>MLRFVTKNSQDKSSDLFSICSDRGTFVAHNRVRTDFKFDNLVFNRVYGVSQKFTLVGNPTVCFNEGSSYLEGIAKKYLTLDGGLAIDNVLNELRSTCGIPGNAVASHAYNITSWRWYDNHVALLMNMLRAYHLQVLTEQGQYS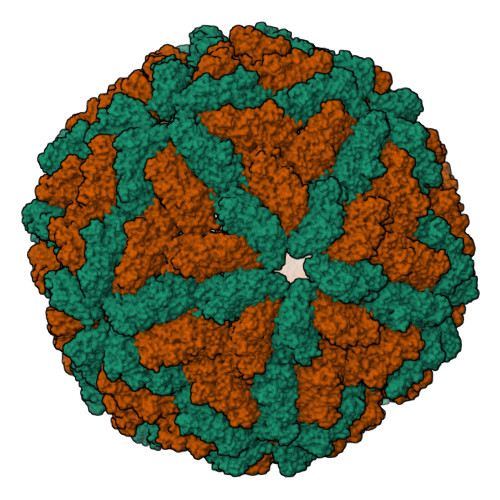AGDIPMYHDGHVKIKLPVTIDDTAGPTQFAWPSDRSTDSYPDWAQFSESFPSIDVPYLDVRPLTVTEVNFVLMMMSKWHRRTNLAIDYEAPQLADKFAYRHALTVQDADEWIEGDRTDDQFRPPSSKVMLSALRKYVNHNRLYNQFYTAAQLLAQIMMKPVPNCAEGYAWLMHDALVNIPKFGSIRGRYPFLLSGDAALIQATALEDWSAIMAKPELVFTYAMQVSVALNTGLYLRRVKKTGFGTTIDDSYEDGAFLQPETFVQAALACCTGQDAPLNGMSDVYVTYPDLLEFDAVTQVPITVIEPAGYNIVDDHLVVVGVPVACSPYMIFPVAAFDTANPYCGNFVIKAANKYLRKGAVYDKLEAWKLAWALRVAGYDTHFKVYGDTHGLTKFYADNGDTWTHIPEFVTDGDVMEVFVTAIERRARHFVELPRLNSPAFFRSVEVSTTIYDTHVQAGAHAVYHASRINLDYVKPVSTGIQVINAGELKNYWGSVRRTQQGLGVVGLTMPAVMPTGEPTAGAAHEELIEQADNVLVE[2x]> GSHMSNKEYRPTLAQLRTFVTIAECKHFGTAATKLSISQPSLSQALVALETGLGVQLIERSTRKVIVTPAGEKLLPFAKSTLDAAESFLSHAKGANGSLTGPLTVGIIPTAAPYILPSMLSIVDEEYPDLEPHIVEDQTKHLLALLRDGAIDVAMMALPSEAPGMKEIPLYDEDFIVVTASDHPFAGRQDLELSALEDLDLLLLDDGHCLHDQIVDLCRRGNINPISSTTAVTRASSLTTVMQLVVAGLGSTLVPISAIPWECTRPGLATANFNSDVTANRRIGLVYRSSSSRAEEFEQFALILQRAFQEAVALAASTGITLK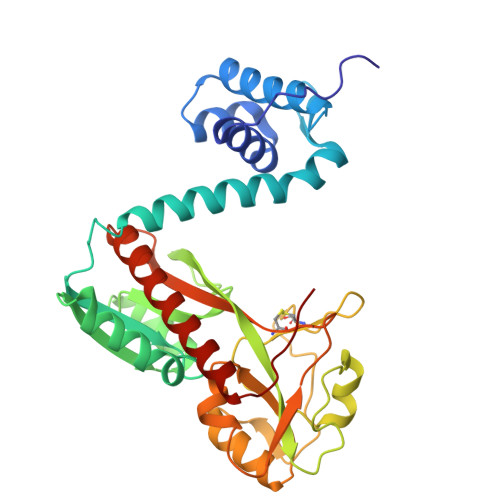QNV> MRITQGTFSFLPDLTDEQIKKQIDYMISKKLAIGIEYTNDIHPRNSFWEMWGLPLFEVTDPAPVLFEINACRKAKSNFYIKVVGFSSERGIESTIISFIVNRPKHEPGFNLIRQEDKSRSIKYSIQAYETYK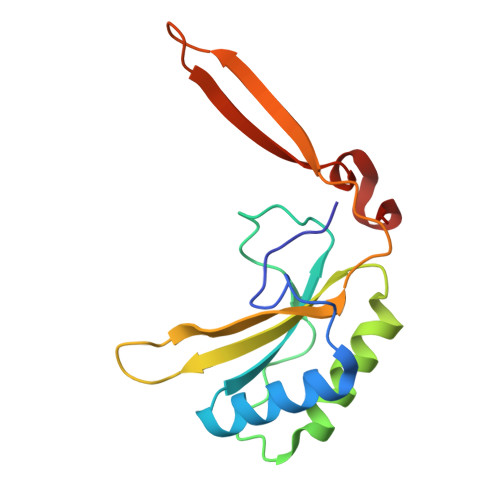PEDQRY> GSHMMFLVVGQGNPGERYARTRHNLGFMVLDRLGLSFRPRGEALVAEAEGGLFLKPLTYYNLTGRAVAPLARFYKIPPERILVVHDEMDLPLGRIRFKAGGSAAGNRGVLSIEEALGTRAFHR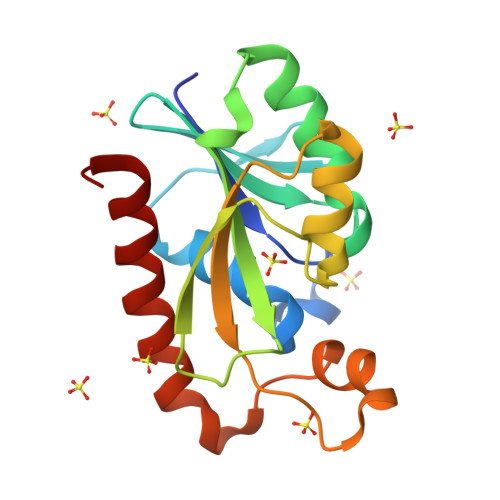LRLGIGKPPDPSRGAEYVLSPFREEELPVVERVLEAAKEAVWCWVREG> GSHMTRETERFPAREFQRDLLDWFARERRDLPWRKDRDPYKVWVSEVMLQQTRYETVIPYFEQFIDRFPTLEALADADEDEVLKAWEGLGYYSRVRNLHAAVKEVKTRYGGKVPDDPDEFSRLKGVGPYTVGAVLSLAYGVPEPAVNGNVMRVLSRLFLVTDDIAKCSTRKRFEQIVR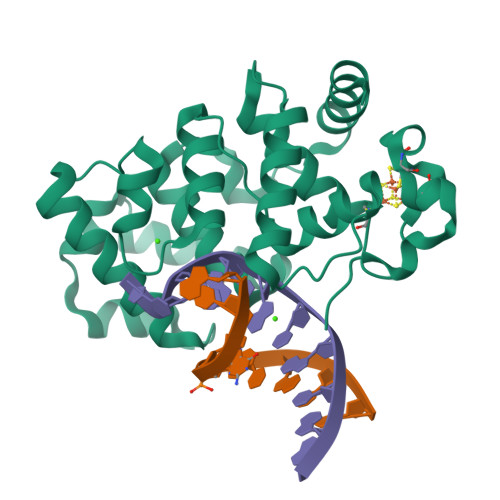EIMAYENPGAFNEALIELGALVCTPRRPSCLLCPVQAYCQAFAEGVAEELPVKM> MILDTDYITENGKPVIRVFKKENGEFKIEYDRTFEPYFYALLKDDSAIEDVKKVTAKRHGTVVKVKRAEKVQKKFLGRPIEVWKLYFNHPQDVPAIRDRIRAHPAVVDIYEYDIPFAKRYLIDKGLIPMEGDEELTMLAFAIATLYHEGEEFGTGPILMISYADGSEARVITWKKIDLPYVDVVSTEKEMIKRFLRVVREKDPDVLITYNGDNFDFAYLKKRCEELGIKFTLGRDGSEPKIQRMGDRFAVEVKGRIHFDLYPVIRRTINLPTYTLEAVYEAVFGKPKEKVYAEEIAQAWESGEGLERVARYSMEDAKVTYELGREFFPMEAQLSRLIGQSLWDVSRSSTGNLVEWFLLRKAYKRNELAPNKPDERELARRRGGYAGGYVKEPERGLWDNIVYLDFRSLYPSIIITHNVSPDTLNREGCKEYDVAPEVGHKFCKDFPGFIPSLLGDLLEERQKIKRKMKATVDPLEKKLLDYRQRLIKILANSFYGYYGYAKARWYCKECAESVTAWGREYIEMVIRELEEKFGFKVLYADTDGLHATIPGADAETVKKKAKEFLKYINPKLPGLLELEYEGFYVRGFFVTKKKYAVIDEEGKITTRGLEIVRRDWSEIAKETQARVLEAILKHGDVEEAVRIVKEVTEKLSKYEVPPEKLVIHEQITRDLRDYKATGPHVAVAKRLAARGVKIRPGTVISYIVLKGSGRIGDRAIPADEFDPTKHRYDAEYYIENQVLPAVERILKAFGYRKEDLRYQKTKQVGLGAWLKVKGKKLEHHHHHH

In this work, we demonstrate these properties using a 9°N DNA polymerase. We show that 3′-esterified dNTP can be incorporated into a template-primer DNA by using MS analysis and X-ray crystallography to validate reaction intermediates and products. We further used structural analyses to examine the incorporation of 3′-NL into DNA.

Before protein crystallization, the incorporation reaction was performed at 4 °C for 16 h with annealed primer-template DNA, dNTP or 3′-NL, and 9°N-I in the presence of Ca2+ (see the Methods section). The DNA with incorporated dAMP is translocated back to the original state, and a divalent ion (Ca2+:1) is near the phosphodiester bond. Similar results were obtained for dTTP, dCTP and dGTP.> TSPAVKRLLGWKQGEQNGQEEKWAEKAVDALVKKLKKKKGAMEELEK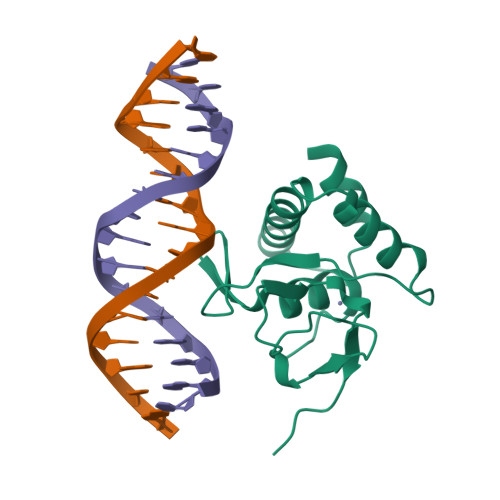ALSSPGQPSKCVTIPRSLDGRLQVSHRKGLPHVIYCRVWRWPDLQSHHELKPLDICEFPFGSKQKEVCINPYHYKRVESPVLPP>[2x]GPDSMPLKRKEEQVDTLICQNLACRATLSLEDGYCKRCSCCICHCYDENKDPSLWLVCNSDPPYLSNSCGMSCHLKCALKHETAGILKNGCYPKLDGSFYCVFCGKVNWLIGSWRKQLLIAKDARRVDVLCDRLSLSHKMLKGTEHYKDMQNIVNTAVKKLKKEVGPLDKVSAVMARGIVNRLNCGTEVQKLCVSAVEAADSMLSSSTD

A PHD finger signature is found in plant vernalization (VEL) proteins, which function as accessory factors of the Polycomb system to control flowering in Arabidopsis through an epigenetic silencing mechanism. During vernalization, VEL proteins associate with Polycomb Repressive Complex 2 and are required for epigenetic silencing of the Arabidopsis FLOWERING LOCUS C (FLC). Here, we use structural analysis by X-ray crystallography to show that the VEL PHD finger forms the central module of a larger compact tripartite superdomain that also contains a zinc finger and a four-helix bundle. Our evidence argues for evolution of a divergent function for the PHD superdomain in vernalization that does not involve histone tail decoding.

We next expressed the equivalent fragment from several other plants species and eventually succeeded in crystallizing the equivalent protein fragment (VIN3123-326) from the palm tree Phoenix dactilyfera (Pd). VIN3123-326 produced diffracting crystals under multiple conditions, whereby the best crystals diffracted to 2.1 Å resolution in space group P3121. VIN3123-326 forms a single compact domain, with an N-terminal ZnF and a C-terminal 4HB, packing tightly against the central PHD module. The topology of the α-helices in 4HB is up-down-up-down, with each helix packing in an antiparallel fashion against the preceding one, thereby forming two straight helical hairpins that associate with each other around a hydrophobic core. The interface between ZnF and PHD finger is relatively small and exhibits only a small number of interactions mediated by water molecules, while that between PHD and 4HB is more extensive and formed by conserved residues engaging in multiple hydrophobic and polar interactions. Notably, one of the key interacting residues in the latter interface is Phe216, the aromatic residue upstream of the final two zinc-coordinating cysteines, which constitutes part of the PHD signature. A striking feature of the VIN3 PHD superdomain is its extensive positive electrostatic surface potential. The positively charged surface patch extending across the Pd VIN3 PHD finger is formed by basic amino acids from each of the three subdomains (R142 and R154 of ZnF; K167 of PHD; R232 and K233 of 4HB). Notably, the long loops in the VEL proteins contain four highly conserved arginine residues (R242, R243, R294, and R299 in Pd VIN3) that are not present in their OBE counterparts. By contrast, we were unable to detect binding of purified PHD superdomain from Phoenix (Pd VIN3123-326) to H3K4me2 nor to other histone H3 tail peptides (methylated or unmodified), including H3K9me2, which was previously reported to be strongly positive for the Arabidopsis PHD domain (see also later).> MIAGQPIFILKEGTKRESGKDAMKENIEAAIAISNSVRSSLGPRGMDKMLVDSLGDIVITNDGVTILKEMDVEHPAAKMMVEVSKTQDSFVGDGTTTAVIIAGGLLQQAQGLINQNVHPTVISEGYRMASEEAKRVIDEISTKIGADEKALLLKMAQTSLNSKSASVAKDKLAEISYEAVKSVAELRDGKYYVDFDNIQVVKKQGGAIDDTQLINGIIVDKEKVHPGMPDVVKDAKIALLDAPLEIKKPEFDTNLRIEDPSMIQKFLAQEENMLREMVDKIKSVGANVVITQKGIDDMAQHYLSRAGIYAVRRVKKSDMDKLAKATGASIVSTIDEISSSDLGTAERVEQVKVGEDYMTFVTGCKNPKAVSILVRGETEHVVDEMERSITDSLHVVASALEDGAYAAGGGATAAEIAFRLRSYAQKIGGRQQLAIEKFADAIEEIPRALAENAGLDPIDILLKLRAEHAKGNKTYGINVFTGEIEDMVKNGVIEPIRVGKQAIESATEAAIMILRIDDVIATKSSSSSSNPPK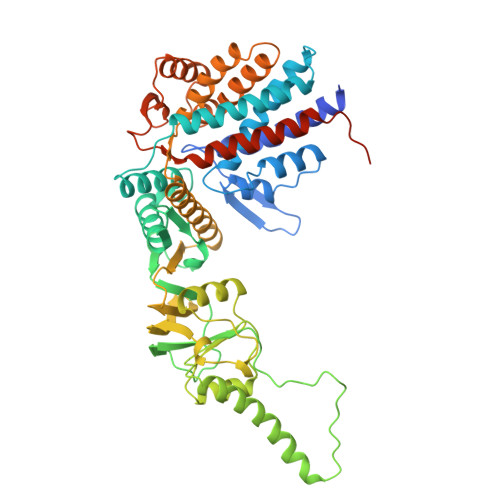SGSSSESSED>[2x]TYTTRQIGAKNTLEYKVYIEKDGKPVSAFHDIPLYADKENNIFNMVVEIPRWTNAKLEITKEETLNPIIQDTKKGKLRFVRNCFPHHGYIHNYGAFPQTWEDPN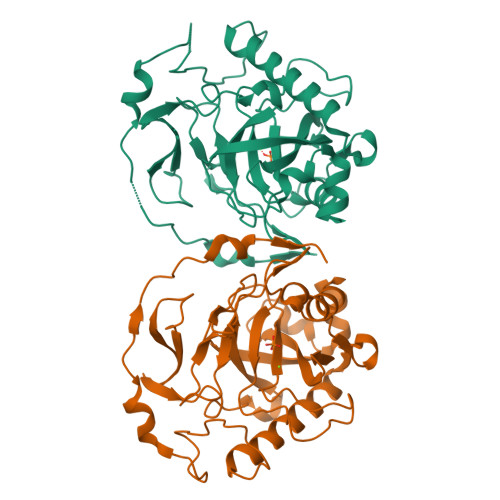VSHPETKAVGDNDPINVLEIGETIAYTGQVKQVKALGIMALLDEGETDWKVIAIDINDPLAPKLNDIEDVEKYFPGLLRATNEWFRIYKIPDGKPENQFAFSGEAKNKKYALDIIKETHDSWKQLIAGKSSDSKGIDLTNVTLPDTPTYSKAASDAIPPASLKADAPIDKSIDKWFFISGSV>SNAMTDDILLIDTDERVRTLTLNRPQSRNALSAALRDRFFAALADAEADDDIDVVILTGADPVFCAGLDLKELAGQTALPDISPRWPAMTKPVIGAINGAAVTGGLELALYCDILIASEHARFADTHARVGLLPTWGLSVRLPQKVGIGLARRMSLTGDYLSATDALRAGLVTEVVAHDQLLPTARRVAASIVGNNQNAVRALLASYHRIDESQTAAGLWLEACAAKQFRTSGDTI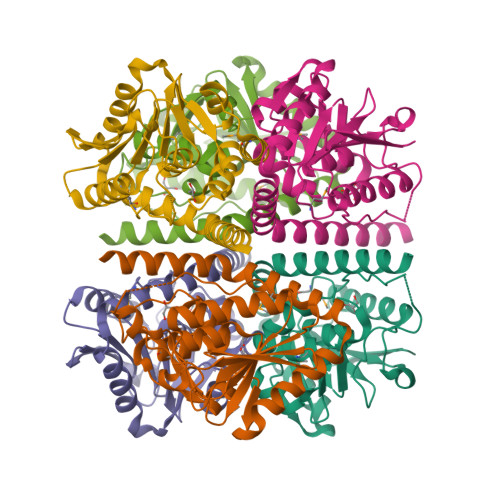AANREAVLQRGRAQVR[3x]>[4x]GAMGSHRSRYFIMLCDNETAIAHAKKTSIWAVKKDSSKRISDAYKKASVYFIFVAQQTYNALG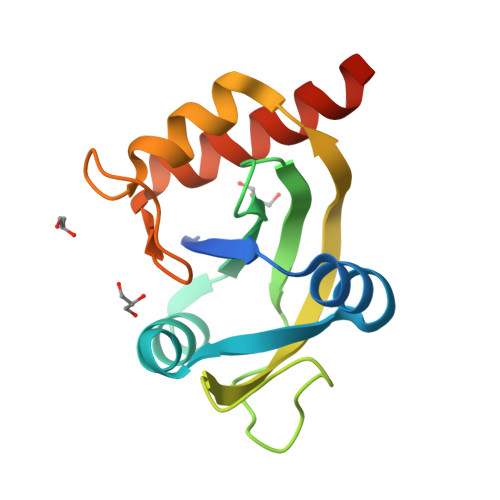YAQVVSDLNSTELPFWSDSSHAGGVRIKWIKTCNLFSAEISEIVSHMDHGSEARDGMEMMYDEGSRLCTLINYAIMKRIGRDR>[2x]MHHHHHHLESSGDFSLLSSPINREKNGTEIVKFSIHPYKGTVIRLGEEILPFKVLEMDKNIALVEMAIPVYKDEKEIELKLSSPGFQNSSYRIRKPEELNEKLIALDKEGITHRFISRFKTGFQPKSVRFIDNTRLAIPLLEDEGMDVLDINSGQTVRLSPPEKYKKKLGFVETISIPEHNELWVSQMQANAVHVFDLKTLAYKATVDLTGKWSKIL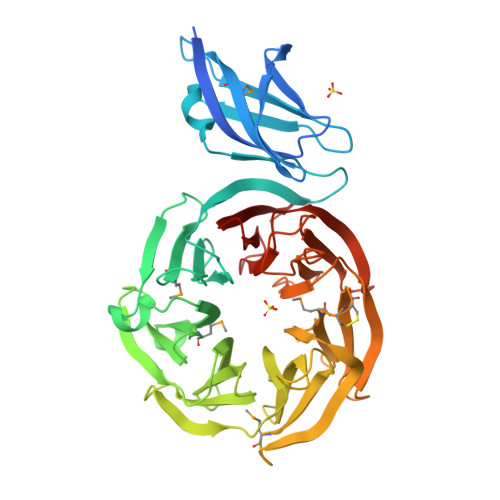LYDPIRDLVYCSNWISEDISVIDRKTKLEIRKTDKIGLPRGLLLSKDGKELYIAQFSASNQESGGGRLGIYSMDKEKLIDTIGPPGNKRHIVSGNTENKIYVSDMCCSKIEVYDLKEKKVQKSIPVFDKPNTIALSPDGKYLYVSCRGPNHPTEGYLKKGLVLGKVYVIDTTTDTVKEFWEAGNQPTGLDVSPDNRYLVISDFLDHQIRVYRRDGF>MHHHHHHGTQQEALGMVETKGLTAAIEAADAMVDSANVMLVGYEKIGSGLVTVIVRGDVGAVKAATDAGAAAARNVGEVKAVHVIPRPHTDVEKILPKGISQ[9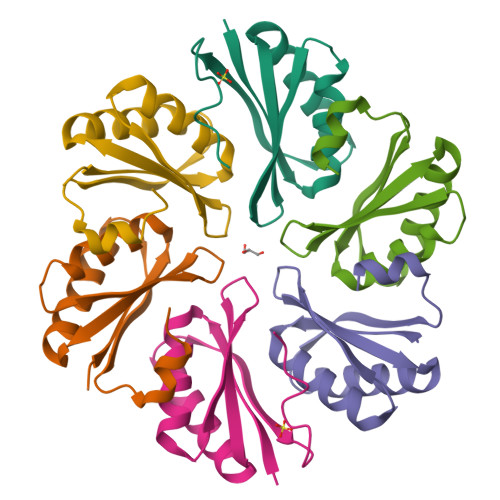x]(2R)-2-azanyl-3-oxidanyl-N-[3-(trifluoromethyloxy)phenyl]propanamide 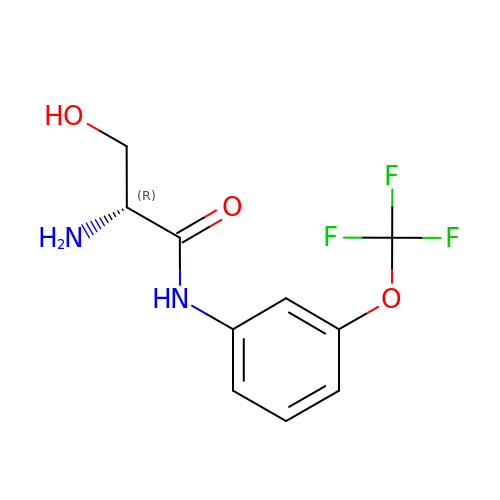| C10 H11 F3 N2 O3 | QKKNXONMXNVCIX-MRVPVSSYSA-N> ATFEIVNRCSYTVWAAASKGDAALDAGGRQLNSGESWTINVEPGTNGGKIWARTDCYFDDSGSGICKTGDCGGLLRCKRFGRPPTTLAEFSLNQYGKDYIDISNIAGFNVPMDFSPTTRGCRGVRCAADIVGQCPAK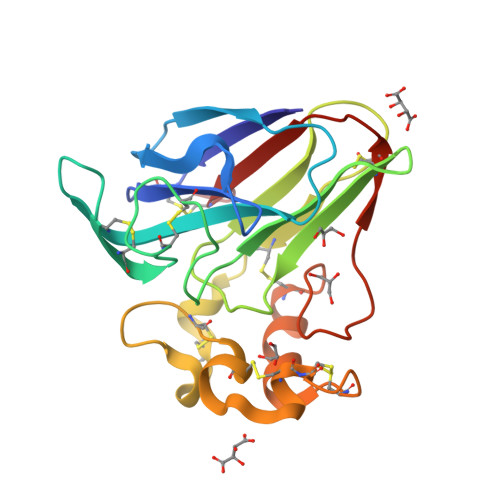LKAPGGGCNDACTVFQTSEYCCTTGKCGPTEYSRFFKRLCPDAFSYVLDKPTTVTCPGSSNYRVTFCPTA>MHHHHHHENLYFQGRFDNKVVVITGAGNGMGEAAARRFSAEGAIVVLADWAKEAVDKVAASLPKGRAMAVHIDVSDHVAVEKMMNEVAEKLGRIDVLLNNAGVHVAGSVLETSIDDWRRIAGVDIDGVVFCSKFALPHLLKTKGCIVNTASQSGLGGDWGAAYYCAAKGAVVNLTRAMALDHGGDGVRINSVCPSLVKTNMTNGWPQEIRDKFNERIALGRAAEPEEVAAVMAFLASDDASFINGANIPVDGGATASDGAPKIV[2x]

In the presence of NADH, acetoin is reduced to 2,3-BDO by the enzyme butanediol dehydrogenase (Bdh). SmBdh exhibits the typical single domain short-chain dehydrogenase/reductase (SDR) architecture. A monomer displays a dinucleotide-binding Rossmann fold that includes seven-stranded parallel β-sheet (β3–β2–β1–β4–β5–β6–β7) flanked by three α-helices (α2, α1, and α8) on one side and three α-helices (α3, α4, and α5) on another. There is an additional small lobe on top of a core structure, formed by two short helices, α6 and α7, creating a deep cleft in which the cofactor is bound, and where the active site is located.

In order to determine the importance of the Gln247 side chain for the catalysis, we developed two mutants of SmBdh: (1) Q247A where this side chain is removed, leaving alanine at position 247 and (2) the double mutant Q247A + V139Q, where the missing glutamine side chain would be reinstated at the position 139 that is present in KpBdh. The SmBdh Q247A and the Q247A + V139Q mutants crystallized in the same space group (P43212) as the WT SmBdh repeating its protein chains arrangement. As with the WT SmBdh, the primary difference between the two molecules in the asymmetric unit in the mutant structures was that molecule A was found in ‘closed’ conformation (that could be best described by ~ 10 Å distance between Cα-atoms of residues Ala93 and Trp192) and molecule B was found in ‘open’ conformation (the corresponding distance is ~ 15 Å). Upon examination of the electron density maps, we were able to locate NAD + cofactor molecule and a substrate in protein molecule A (‘closed’ conformation), whereas in molecule B (‘open’ conformation) the corresponding space is occupied by only adenine diphosphate (as in Q247A mutant) or remains unoccupied (as in Q247A + V139Q mutant) at all. In the Q247A + V139Q double mutant structure, an ethylene glycol molecule was modeled at the substrate-binding pocket. As with the Q247A mutant, acetoin was present during crystallization, but raising its concentration was damaging to the crystals. We suggest that the available space in the substrate binding site became reduced compared to the Q247A single mutant, thereby providing insufficient space for glycerol to fit. Instead, ethylene glycol which is comparable in size to acetoin could fit. In comparison to the WT SmBdh, Q247A mutant showed a ~ 90% loss in activity as predicted by the structure, whereas the double mutant Q247A + V139Q showed ~ 300% improvement in activity in comparison to Q247A mutant. Although the double mutant did not completely restore the loss of Gln247 activity, significant function was regained by introducing the V139Q mutation in this protein.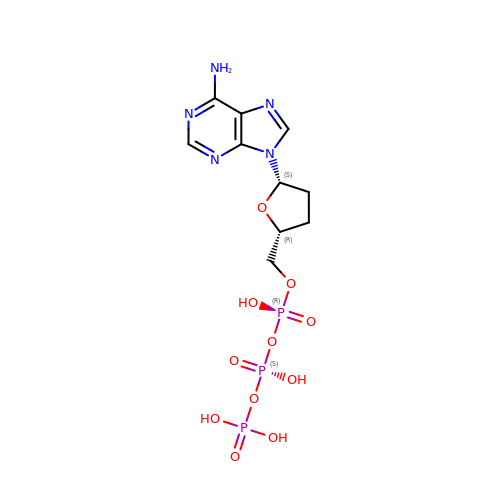2',3'-DIDEOXYADENOSINE-5'-TRIPHOSPHATE | C10 H16 N5 O11 P3 | OAKPWEUQDVLTCN-RQJHMYQMSA-N>ILQTTVDGNSTAISNLKSDISSNGLAITDLQDRVKSLESTASHGLSFSPPLSVADGVVSLDMDPYFCSQRVSLTSYSAEAQLMQFRWMARGTNGSSDTIDMTVNAHCHGRRTDYMMSSTGNLTVTSNVVLLTFDLSDITHIPSDLARLVPSAGFQAASFPVDVSFTRDSATHAYQAYGVYSSSRVFTITFPTGGDGTANIR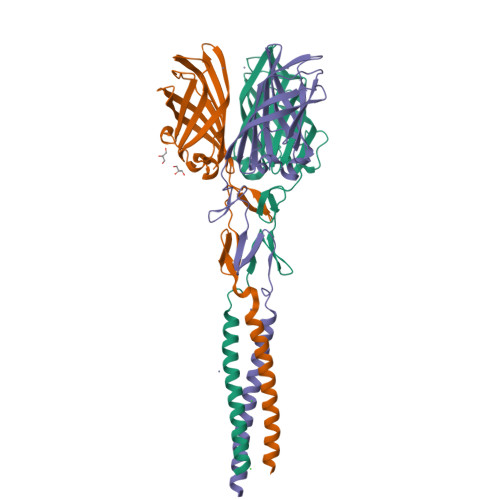SLTVRTGIDT[3x]>[2x]TNTDSFTFSKFKPNQPNLKKQGDATVTSSGTLQLTKVDKNGVPDPKSLGRALYASPINIWDSKTGVVASFATSFRFTIYAPNIATIADGLAFFLAPVSSPPKAGAGFLGLFDSAVFNSSYQTVAVEFDTYENTVFLDPPDTHIGIDVNSIKSIKTVKWDLANGEAAKVLITYDSSAKLLVAALVYPSSKTSFILSDVVDLKSVLPEWVSIGFSAATGASSGYIETHDVFSWSFASKLSFXXXXXXLDLASFLVAN;>TNTDSFTFSKFKPNQPNLKKQGDATVTSSGTLQLTKVDKNGVPDPKSLGRALYASPINIWDSKTGVVASFATSFRFTIYAPNIATIADGLAFFLAPVSSPPKAGAGFLGLFDSAVFNSSYQTVAVEFDTYENTVFLDPPDTHIGIDVNSIKSIKTVKWDLANGEAAKVLITYDSSAKLLVAALVYPSSKTSF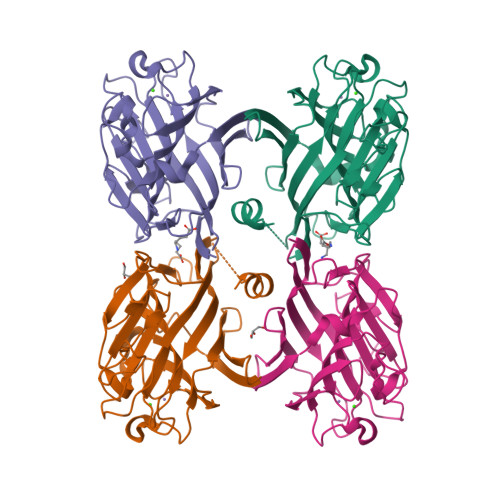ILSDVVDLKSVLPEWVSIGFSAATGASSGYIETHDVFSWSFASKLSF[2x];>AEETSFVFSKFKPLEPNLILQGDALVTVAGVLQLTNVDKNGVPEPSSLGRATYSAPINIWDSATGLVASFATSFRFTIYAPNIATIADGLAFFLAPVASAPDSGGGFLGLFDSAVSGSTYQTVAVEFDTYENTVFTDPPYTHIGFDVNSISSIKTVKWSLANGEAAKVLITYNSAVKLLVASLVYPSSKTSFILADIVDLSSVLPEWVRVGFSAATGASGGKIETHDVFSWSFASKLAGXXTKDSSFLDGG[2x];>AEETSFVFSKFKPLEPNLILQGDALVTVAGVLQLTNVDSNGVPEPSSLGRATYSAPINIWDSATGLVASFATSFRFTIYAPNIATIADGLAFFLAPVASAPDSGGGFLGLFDSAVGDTTYQTVAVEFDTYENTVFTDPPYTHIGFDVNSISSIKTVKWSLANGEAAKVLITYNSAVKLLVASLVYPSSKTSFILADIVDLSSVLPEWVRVGFSAATGASKGYIETHDVFSWSFASKLAG[2x]> MGTGKELVLALYDYQ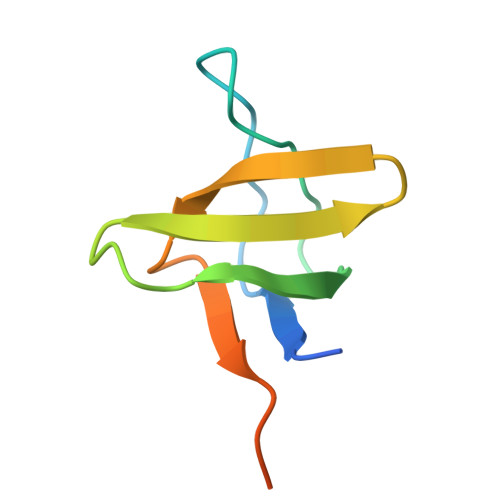EKSPREVTMKKGDILTLLNSTNKDWWKVEVNDRQGFVPAAYVKKLDPAQSASRENLGG> MDDMVLVLARNLSGKAKGKPAPKGAPAPPPPPVASSAVTANPATRSAGARIRRNQPRLDPLTLLTPQQRELAESLAHLSRQAAQPPSATAAGADALTPAAEAAADAAAEAAAAPLRGLGEVPLPLRRREVAALVDAALTGAAGGQQVHFQPFVFNDIFQSAPAAATYVAEALESGSAWGRIERFFLAAAEADAG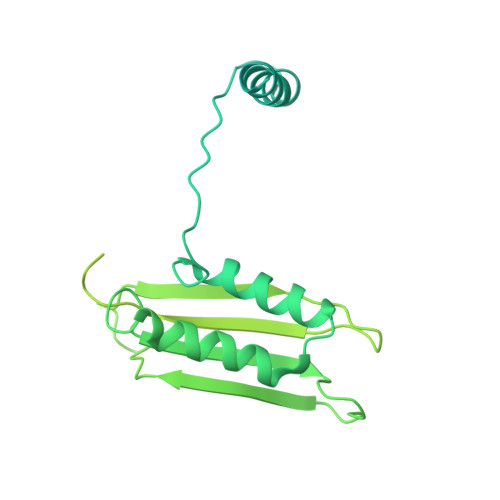KLVAAVRVEVAGRIGRKADMAATKSWAWGDLRLASLTSKLDYGTAAANTRMGVLGIKVWIRYQPAAAPDLYFPATGGSGLHAPLPAGAAPSMSLDELYAAALERSGSSSSSSSSSSVGGAGGSSTRYGAVGWWSRPAGQQPAANRVHEVFTPEFNPKAGDRLDGYLRRAAESRRVFRSAANREEYMATVGRFLVKQRQAAKARAAAEAYAAALSATKPATIPTTSSSSSSSSANSSAASSVPARPRLGRRPHRPLARFPVEAFSPLGRRGPVLLRWRLQAAAAVGKGKGGNGERRA>MPIIERIQAREILDSRGNPTVQVEVTTDYEITGVANVPSGASTGSREALELRDKGTKYEGNWFGGKGVMTAVDNVNEKIAPELIGMSVFDQRAIDKLMIELDGTATKSKLGANAILGVSLAVARAAATELGMPLYRYIGGANAHTLPLPMLNVLNGGEHASNTVDFQEFMIMPVGAKSLREALQMANKVFHNLAKLLKKAGYGTQVGDEGGFAPNCKSHEEVLDYLVEAIKVAGYTPATSGKNAIAIALDAACSELYDENSKKYTFKKLKQAIAEKRSGFEHLDNVKLEYTTDELIEYFGKLIDKYPIISIEDGLAESDWEGFAKMTAKFGSKVQIVGD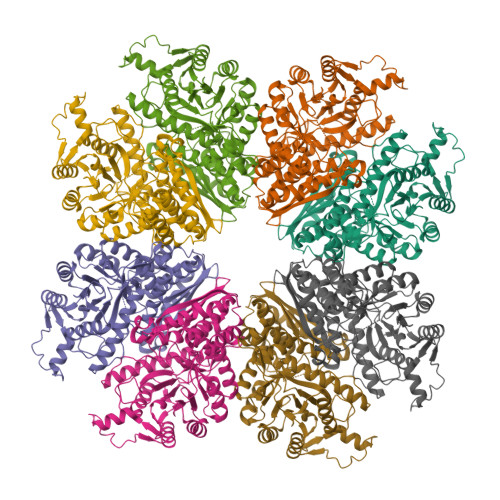DLTVTNPKLLEKAIEQKSMNAILIKLNQIGSLSETMDAINKAQKANMACVVSHRSGETEDTTIADLAVAFNTGQIKTGSMSRTDRIAKYNRLLVIEEELGEQSEFEGSKAFYNIKLEHHHHHH[2x]methyl 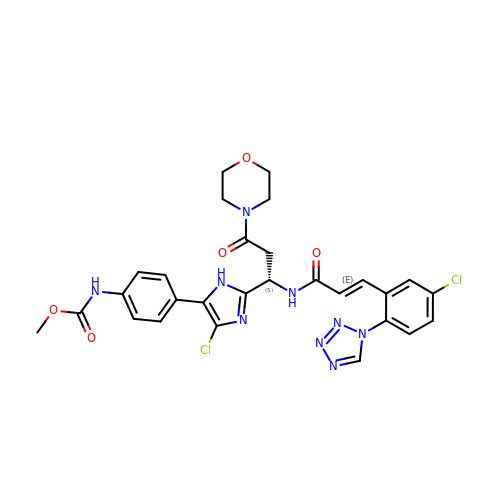(4-{4-chloro-2-[(1S)-1-({(2E)-3-[5-chloro-2-(1H-tetrazol-1-yl)phenyl]prop-2-enoyl}amino)-3-(morpholin-4-yl)-3-oxopropyl]-1H-imidazol-5-yl}phenyl)carbamate | C28 H27 Cl2 N9 O5 | JXLVPHOTGHZUCE-ZSIUJALASA-N> MSLRRGIYHIENAGVPSAIDLKDGSSSDGTPIVGWQFTPDTINWHQLWLAEPIPNVADTFTLCNLFSGTYMDLYNGSSEAGTAVNGWQGTAFTTNPHQLWTIKKSSDGTSYKIQNYGSKTFVDLVNGDSSDGAKIAGWTGTWDEGNPHQKWYFNRMSVSSAEAQAAIARNPHIHGTYRGYILDGEYLVLPNATFTQIWKDSGLPGSKWREQIYDADDFAIAMKAAVGKWGADSWKANGFAIFCGVMLGVNKAGDAAAAYNFTLTKDHADIVFFEPQNGGYLNDIGYDSYMAFY;> PVVR

The Marasmius oreades agglutinin (MOA) is the holotype of an emerging family of fungal chimerolectins and an active Ca2+/Mn2+-dependent protease, which exhibits a unique papain-like fold with special active site features. While acting as a dimerization domain, the papain-like domain of MOA retains the characteristic L-/R-domain partition of PLCPs. As additional feature, the MOA dimer carries two binuclear metal-binding clusters, symmetrically placed at the dimerization interface (Grahn et al., 2009). MOA requires the presence of calcium or manganese (II) to switch from the inactive form to an active protease (Cordara et al., 2011, Wohlschlager et al., 2011).

In an effort to validate our substrate binding model, we co-crystallized the enzymatically inactive MOA variants C215A and C215A/H257A with two synthetic heptapeptides mimicking proteolytic substrates. The designed peptides have the sequence PVxRAHS (with x = P or V). (2016) for subsites S4–S1 and S1′-S3′. The P2 (‘x’) position is occupied by either a proline or a valine residue to address the MOA S2 specificity pocket preference for both amino acids. To our surprise, the co-crystallized peptide probes were cleaved in both structures, despite the fact that we used catalytically inactive enzymes. The observed cleavage products correspond to the N-terminal proteolytic fragments, binding to the MOA active site in the standard backbone orientation expected for PLCP substrates. The synthetic peptides are anchored to the active site through three main contact points: the oxyanion hole, defined by Trp208 and the backbone NH group of Ala215, the ‘site B’ Ca2+ ion and a backbone–backbone interaction with Ala256. The presence of an arginine residue at the P1 position unambiguously maps the S1 subsite to the carboxylate group of L-domain Glu210, which forms a side-on bidentate salt bridge with the Arg guanidinium group. The P2 moiety binds to the S2 specificity pocket lined by residues Leu247, Ala258 and Leu182# (with ‘#’ identifying a residue provided by the other subunit). Substitution of Pro for Val at the P2 position yields a minor conformational change at the P3 and P4 positions of the peptides, and a lower occupancy of the bound proteolytic fragment.> LPPEAIKQPSPTKVELVVGELASIKFDNSVLVNPANAQLTNGGGAARAIAKLAGPKYQEYCNSVAPISGPLTTDSFDAKKLGVACILHVVPPKGSDPNVQELLYQAYKSILTEPAHYVIPILGAGIFGCNPVHSLDAFRKACPSDIGRVTLVTMNKNHLQVWDALNRTIVRTTTDYD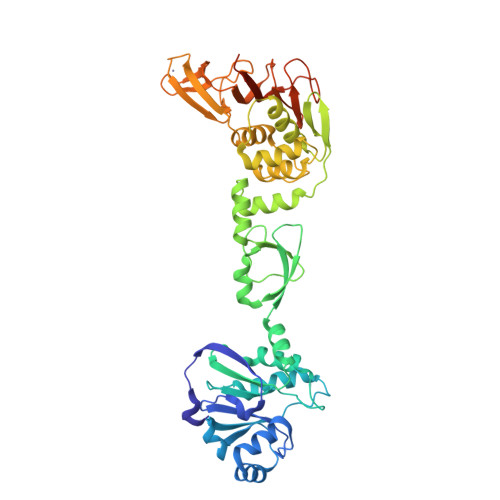QVTTKALTPQGVLEANLFDGEDFVQEPKPGQIYLEVTEEVQNQAKELDLNLQQYCVYLKTCHHKWVVSRTNGLMHLKQKDNNCFVSAGVNLFQNTAYQFRPAIDALYREYLNGNPNRFVAWIYASTNRRVGEMGCPQQVISLLVSNSDAAFSATTACCNTYFNHTGVISVAREYDPIQPKVYCMKCDVWTPFTPQSGKGAVAIGTSADEPTGPAIKFAAAHCWYTNGKKTVNGYDTKANVVATYHRFDVPKPQLVEDVVALPTKNDFEHHHHHH>[2x]SNAMTSS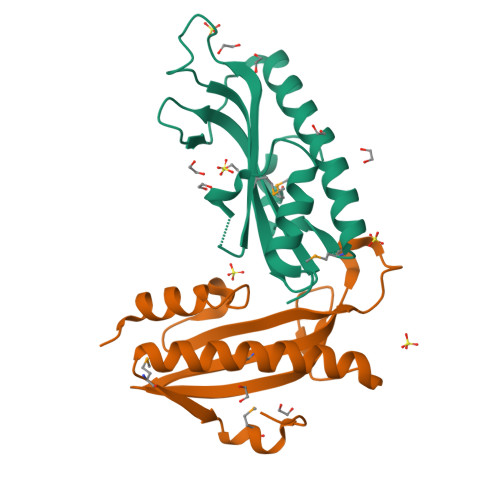LHPTRGKLLKRFAQIGPYIREQQCQESQFFFDCLAVCVNKKVTPEKREFWGWWMELERNGEQLIYYYQVGLFDKNGDWVNQVISKKDVIESIHETLIRFHDFLQAAVSELEMTLVPDEKMSNFPLPL> DFPNNKETGEALLTPVDATASSHDGNGPDRLIDQDLTTRWSSAGDGEWAMLDYGSVQEFDAVQASFSKGNERQSKFDIQVSVDGETWTTVLENQLSSGKAIGLERFQFEPAVKARYVRYVGHGNTKNGWNSVTGLAAVNCSINACPASQIITSDVVAAEAVLIAEMKAAEKARKAARKDLRSGNFGVAAVYPCETSVKCDTRSALPVPTGLPATPVAGNAPSENFDMTHWYLSQPFDHDKNGKPDDVSEWNLANGYQHPEIFYTADDGGLVFKSYVKGVRTSKNTKYARTELREMMRRGDQSISTKGVNKNNWVFSSAPEADLEAAAGIDGVLEATLKIDHATTTGNANEVGRFIIGQIADQNDEPIRLYYRKLPNQPTGAVYFAHESQDATKEDFYPLVGDMTAEVGEDGIALGEVFSYRIDVKGNTMTVTLMREGKDDVVQVVDMSNSGYDVGGKYMYFKAGVANQNISGDLDDYSQATFYQLDVSHDQYKK

In heterotrophic bacteria that use alginates as crucial nutrients, alginate lyases depolymerize alginate into alginate oligosaccharides (AOSs) and then into monomers for assimilation into the central metabolism. The overall structures of these PL7 alginate lyases are similar, showing a β-jelly roll fold composed of two antiparallel β-sheets with a deep cleft. The noteworthy structural differences among the solved PL7 structures are the loops around the deep cleft, which are variable in length and sequence and involved in alginate substrate binding with the deep cleft. Structural study on several PL7 alginate lyases reveals that two loops around the substrate binding cleft determine product distribution.

In a previous study, we reported a multidomain alginate lyase AlyB, which contained CBM32 (a carbohydrate binding domain) and a PL7 catalytic domain (named CD2AlyB). One intriguing feature of AlyB is that its CBM32 had little effect on enzymatic activity but rather specified that trisaccharides were predominant in the degradation products when these two domains were combined with an alpha helix linker. To explore the substrate binding profile of AlyB, we screened the crystals of the AlyB-substrate complex using the noncatalytic mutant AlyBH360A_Y466A (His360 and Tyr466 are conserved catalytic residues) and the substrate G9 (GGGGGGGGG). Surprisingly, the structure of AlyBH360A_Y466A-G9 complex was solved at a resolution of 2.25 Å, binding the longest substrate among all solved alginate lyase structures and providing the substrate binding profile from subsite -3 to subsite +6. Structural comparison demonstrated that there was a clear linker twist that occurred upon G9 binding, which not only shortened the distance between CBM32 and CD2AlyB but also enabled the ligand-binding region of CBM32 to turn toward the end of the “-” section of CD2AlyB, effectively blocking sugar extension. Analysis of the detailed interactions between AlyB and G9 indicated that a total of seven residues from CBM32 were involved in substrate binding, of which six residues formed hydrogen bonds and Trp129 formed hydrophobic contact, and more interestingly, they all formed interactions with the sugar unit at subsite -3. In contrast, only three residues from CD2AlyB participated in substrate binding at subsites -2 and -1. For substrate binding at the “+” section, the conserved residues in the PL7 family (corresponding to Arg289, Arg293 and Gln358 in AlyB) also formed interactions with the C-5 carboxyl group at subsites +1, +2 and +3, and a similar substrate binding profile was observed after structural comparison of the AlyBH360A_Y466A-G9 complex and the A1-II’-GGMG complex. Additionally, the “-” section of CD2AlyB accommodated exactly three sugar units because of the blocking effect produced by CBM32, which led to trisaccharide release during substrate degradation.> MSGDENPASKPTPVQDVQGDGRWMSLHHRFVADSKDKEPEVVFIGDSLVQLMHQCEIWRELFSPLHALNFGIGGDSTQHVLWRLENGELEHIRPKIVVVWVGTNNHGHTAEQVTGGIKAIVQLVNERQPQARVVVLGLLPRGQHPNPLREKNR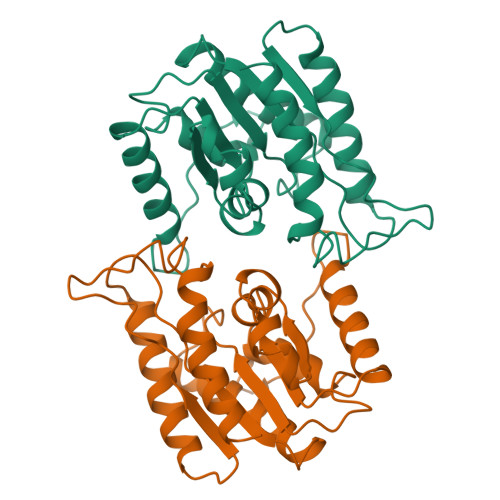RVNELVRAALAGHPRAHFLDADPGFVHSDGTISHHDMYDYAHLSRLGYTPVCRALHSLLLRLLTQDQGQGGAPLPEPSPP> QQKKNLSFTNP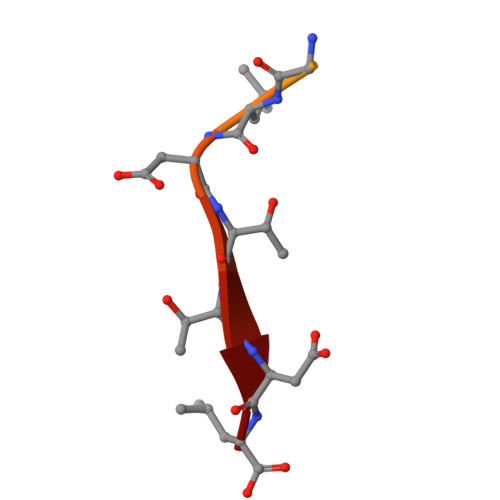GLDTTDL>[4x]SHHHHHHSSGLVPRGSHMNNSQLAGKRILVTQADTFMGPTLCEVFAEMGAEVIAD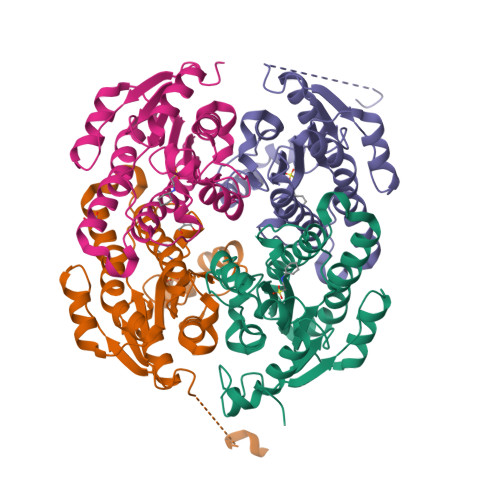NNLLTDPALPAKIIQQAGHIDVLVINLAIPAPFTKGELVDDSEWSATFSAVVDPMPRLCTAVLPQMIERQGGKILVMGSASALRGMKRASTYSAARGAQLSYVKAMGVEMAPQGIQINAIAQNFVDNPTYFPEETKANPKFQERLKRDVPLGRLVSLREDALFAAYLCSDAADCFVGQVFPVSGGWAV> MGSVTPIPLPKIDEPEEYNTNYILFWNHVGLELNRVTHTVGGPLTGPPLSARALGMLHLAIHDAYFSICPPTDFTTFLSPDTENAAYRLPSPNGANDARQAVAGAALKMLSSLYMKPVEQPNPNPGANISDNAYAQLGLVLDRSVLEAPGGVDRESASFMFGEDVADVFFALLNDPRGASQEGYHPTPGRYKFDDEPTHPVVLIPVDPNNPNGPKMPFRQYHAPFYGKTTKRFATQSEHFLADPPGLRSNADETAEYDDAVRVAIAMGGAQALNSTKRSPWQTAQGLYWAYDGSNLIGTPPRFYNQIVRRIAVTYKKEEDLANSEVNNADFARLFALVDVACTDAGIFSWKEKWEFEFWRPLSGVRDDGRPDHGDPFWLTLGAPATNTNDIPFKPPFPAYPSGAATFGGAVFQMVRRYYNGRVGTWKDDEPDNIAIDMMISEELNGVNRDLRQPYDPTAPIEDQPGIVRTRIVRHFDSAWELMFENAISRIFLGVHWRFD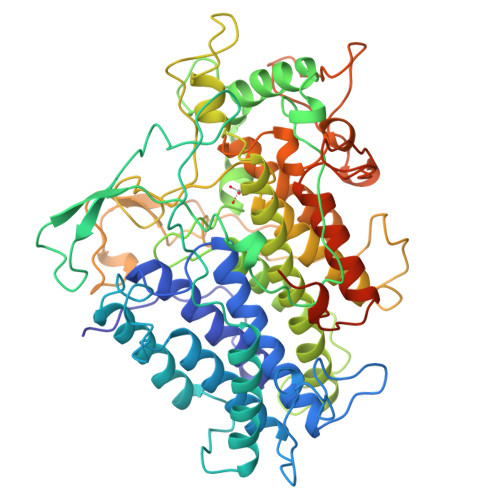AAAARDILIPTTTKDVYAVDNNGATVFQNVEDIRYTTRGTREDEEGLFPIGGVPLGIEIADEIFNNGLKPTPPEIQPMPQETPVQKPVGQQPVKGMWEEEQAPVVKEAP8-(1-methyl-1H-imidazol-4-yl)-2-(4,4,4-trifluorobutoxy)pyrido[3,4-d]pyrimidin-4-ol | C15 H14 F3 N5 O2 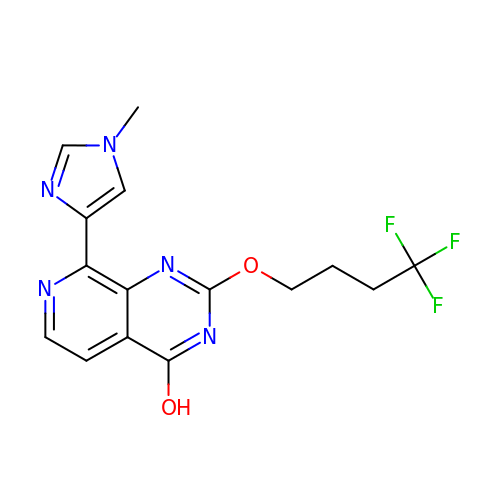| GVIVKUKLHYWHES-UHFFFAOYSA-N> MRLFVSDGVPGCLPVLAAAGRARGRAEVLISTVGPEDCVVPFLTRPKVPVLQLDSGNYLFSTSAICRYFFLLSG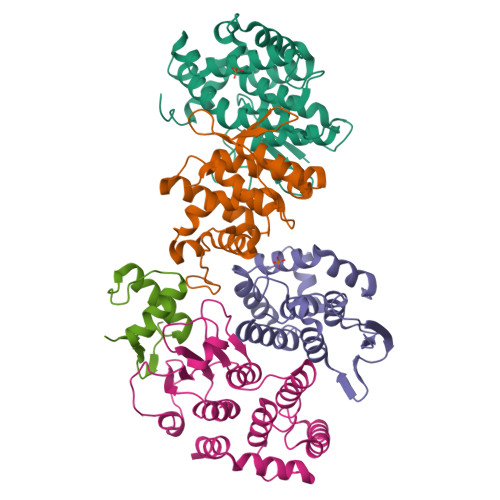WEQDDLTNQWLEWEATELQPALSAALYYLVVQGKKGEDVLGSVRRALTHIDHSLSRQNCPFLAGETESLADIVLWGALYPLLQDPAYLPEELSALHRWFQTLSTQEPCQRAAETVLKQQGVLALRPYLQKQPQPSPAEGRAVTNEPEEEELEHHHHHH;> MRGSHHHHHHGSMAAAAELSLLEKSLGLSKGNKYSAQGERQIPVLQTNNGPSLTGLTTIAAHLVKQANKEYLLGSTAEEKAIVQQWLEYRVTQVDGHSSKNDIHTLLKDLNSYLEDKVYLTGYNFTLADILLYYGLHRFIVDLTVQEKEKYLNVSRWFSHIQHYPGIRQHLSSVVFIKNRLYTNSH;> MATLSLTVNSGDPPLGALLAVEHVKDDVSISVEEGKENILHVSENVIFTDVNSILRYLARVATTAGLYGSNLMEHTEIDHWLEFSATKLSSSDSFTSTINELNHSLSLRTYLVGNSLSLADLSVWATLKGNAAWQEQLKQKKAPVHVKRWFGFLEAQQAFQSVGTKWDVSTTKAR;> MTNIIQADEPTTLTTNALDLNSVLGKDYGALKDIVINANPASPPLSLLVLHRLLCEHFRVLSTVHTHSSVKSVPENLLKCFGEQNKKQPRQDYQLGFTLIWKNVPKTQMKFSIQTMCPIEGEGNIARFLFSLFGQKHNAVNATLIDSWVDIAIFQLKEGSSKEKAAVFRSMNSALGKSPWLAGNELTVADVVLWSVLQQIGGCSVTVPANVQRWMRSCENLAPFNTALKLLKLEHHHHHH;> MGSSHHHHHHSSGLVPRGSHMPSASASRKSQEKPREIMDAAEDYAKERYGISSMIQSQEKPDRVLVRVRDLTIQKADEVVWVRARVHTSRAKGKQCFLVLRQQQFNVQALVAVGDHASKQMVKFAANINKESIVDVEGVVRKVNQKIGSCTQQDVELHVQKIYVISLAEPRLPLQLDDAVRPEAEGEEEGRATVNQDTRLDNRVIDLRTSTSQAVFRLQSGICHLFRETLINKGFVEIQTPKIISAASEGGANVFTVSYFKNNAYLAQSPQLYKQMCICADFEKVFSIGPVFRAEDSNTHRHLTEFVGLDIEMAFNYHYHEVMEEIADTMVQIFKGLQERFQTEIQTVNKQFPCEPFKFLEPTLRLEYCEALAMLREAGVEMGDEDDLSTPNEKLLGHLVKEKYDTDFYILDKYPLAVRPFYTMPDPRNPKQSNSYDMFMRGEEILSGAQRIHDPQLLTERALHHGIDLEKIKAYIDSFRFGAPPHAGGGIGLERVTMLFLGLHNVRQTSMFPRDPKRLTP> MAEVISISNATRVHSYRGVLIITDELTVEA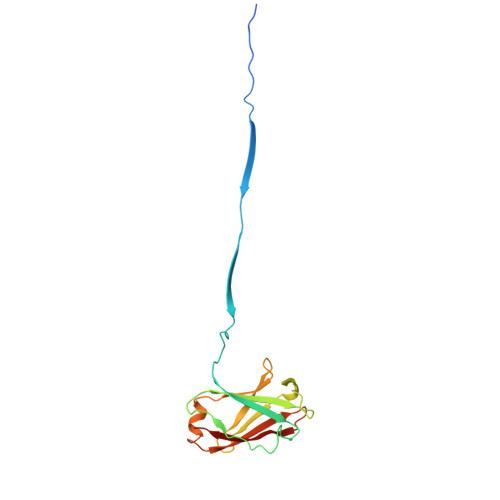GSRVSLSGYVSDGGTSDVFTICRLLDAPMNGKQFISNNCNEIVKIPFDSSCLLGVKLYNCENKRVNVNSVEAAFITIDTAFQSPMTVNKESNRLEYIFSQNDYKVLVKGKVYDMIVNVVDESGNHSTILKQKVRFN> GPHMPGSGQIQLWQFLLELLSDSANASCITWEGTNGEFKMTDPD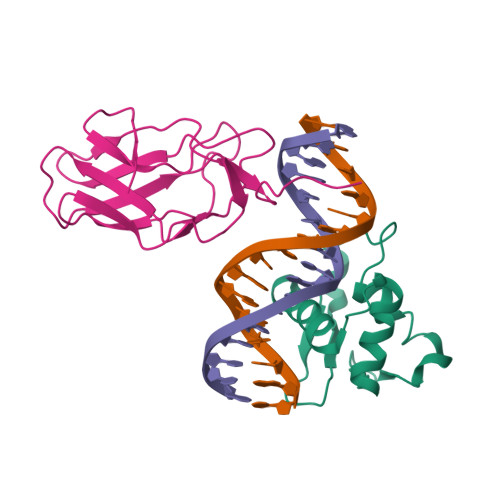EVARRWGERKSKPNMNYDKLSRALRYYYDKNIMTKVHGKRYAYKFDFHGIAQALQPHPTE;> AELVRTDSPNFLCSVLPSHWRCNKTLPVAFKVVALGEVPDGTVVTVMAGNDENYSAELRNASAVMKNQVARFNDLRFVGRSGRGKSFTLTITVFTNPPQVATYHRAIKVTVDGPREPRRHRQK>MEPTTEIQATEDLTLSGDHAAASADSLVVDNANDNAGQEEGFEIVLKDDETAPKQDPAKNAEFARRRIERKRQRELEQQMEAVKRGELPESLRVNPDLPPQPDINAYLSEEGLAKYDYDNSRALA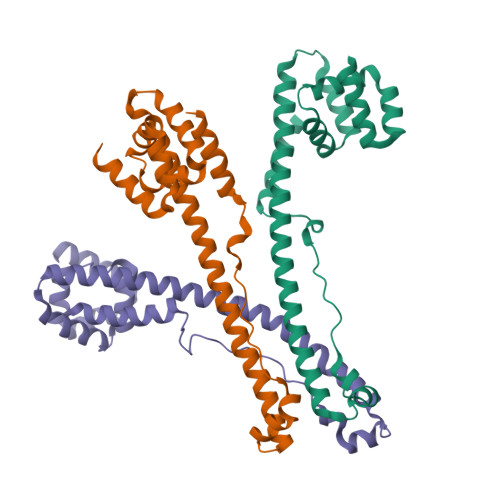AFNAANTEWLMKAQDARSNAVAEQGRKTQEFTQQSAQYVEAARKHYDAAEKLNIPDYQEKEDAFMQLVPPAVGADIMRLFPEKSAALMYHLGANPEKARQLLAMDGQSALIELTRLSERLTLKPRGKQISSAPPADQPITGDVSAANKDAIRKQMDAAASKGDVETYRKLKAKLKGIR[3x]>[2x]GSESPAAPPTTAPPPHVIIVPSAGMGHLIPLAEFAKRLLPRFTFTFAVPTSGPPSSSQRDFLSSLPASIDTSFLPEVDLSDAPSDAQIETLMSLMVVRSLPSLRDLIASYSASGRRVAALVVDLFATDAIDVALELGIRPFIFFPSTAMTLSFF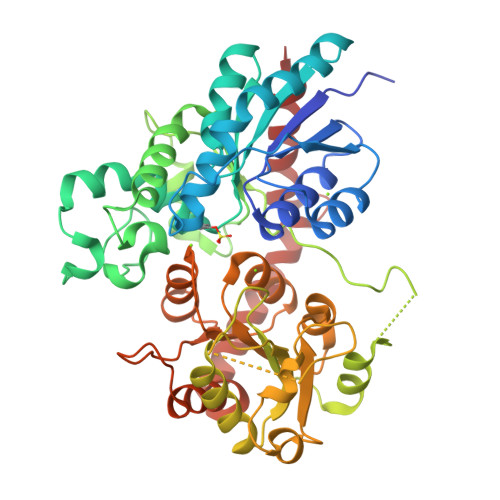LHLEKLDETVSCEFAELSDPVQIPGCIPVHGKDLIDPVQDRKNDAYKWLLHHSKRYKLAEGVIVNSFEGLEGGPIRELLHPEPGKPRVYPVGPLIQAGSCEKGAAARPECLKWLDQQPRGSVLFVNFGSGGVLSTEQQNELAGVLAHSQQRFLWVVRPPNDGIANATYFSVDGEIDPLKLLPEGFLEQTAGRGLVLPMWAPQIDVLSHESTGGFLTHCGWNSTLESVFHGVPLITWPLYAEQKMNAVMLTEGLRVGLRPSVGKDGIIRGAEIARVIGELMEGEEGKRIRSKMQELKRAASAVLSKDGSSTRALEEVAKIWESKV> MGLLDRLSGLLGLKKKEVHVLCLGLDNSGKTTIINKLKPSNAQSQDIVPTIGFSIQK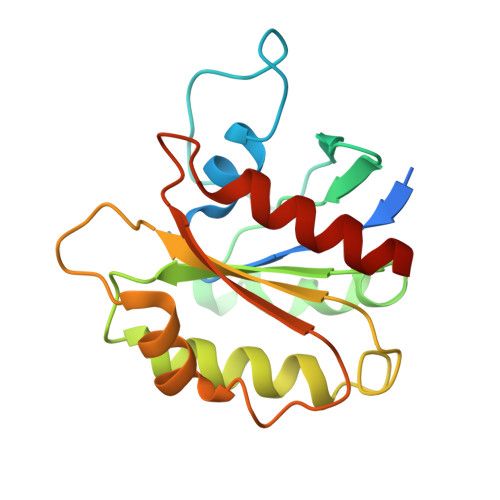FKSSSLSFTVFDMSGQGRYRNLWEHYYKEGQAIIFVIDSSDKLRMVVAKEELRTLLNHPDIKHRRIPILFFANKMDLRDALTSVKVSQLLCLEDIKDKPWHICASDAIKGEGLQEGVDWLQDQIQSVKT(2~{S})-2-[(~{E})-[2-methyl-3-oxidanyl-5-(phosphonooxymethyl)pyridin-4-yl]methylideneamino]-3-oxidanylidene-propanoic acid | C11 H13 N2 O8 P | 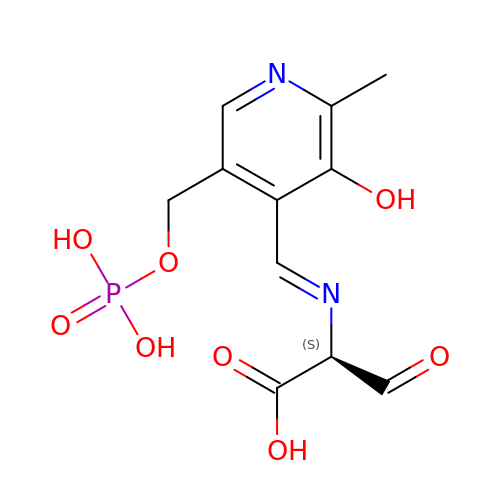GAMDABAFAVQUPR-BIMOUXMDSA-N>SLNTDDIQGDILVGMHKQKQLFYFFAINDPATFKTHLASDIAPVVASVTQLSNVATQPLVALNIAFSNTGLLALGVTDNLGDSLFANGQAKDATSFKESTSSWVPQFAGTGIHGVIILASDTTDLIDQQVASIESTFGSSISKLYSLSASIRPGNEAGHEMFGFLDGIAQPAINGFNTPLPGQNIVDAGVIITGATNDPITRPSWAVGGSFLAFRQLEQLVPEFNKYLLDNAPAGSGSLQARADLLGARMVGRWKSGAPIDLTPTADDPALGADAQRNNNFTYSHAGFDLGSDQSHCPFSAHIRKTRPRA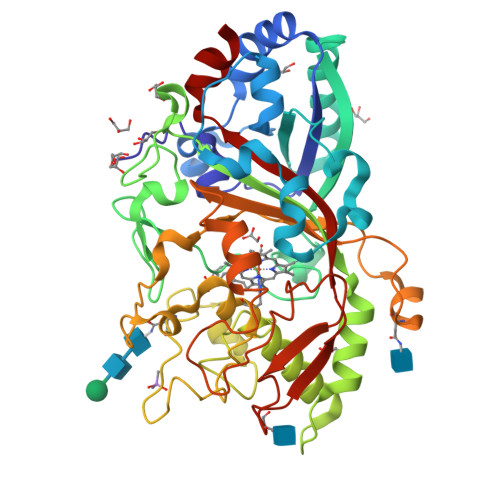DLGGSLTPPNLSAGANSIMRSGIPYGPEVTSAESASNTTTQERGLAFVAYQAQLSQGFHFLQQTWADNANFPPGKTPATVGLDPIIGQNNGQPRVVNGLLPSNSSASLSIPQFVVSHGGEYFFSPPISAIGGRLSA[2x]> DSLDEQRSRYAQIKQAWDNRQMDVVEQMMPGLKDYPLYPYLEYRQITDDLMNQPAVTVTNFVRANPTLPPARTLQSRFVNELARREDWRGLLAFSPEKPGTT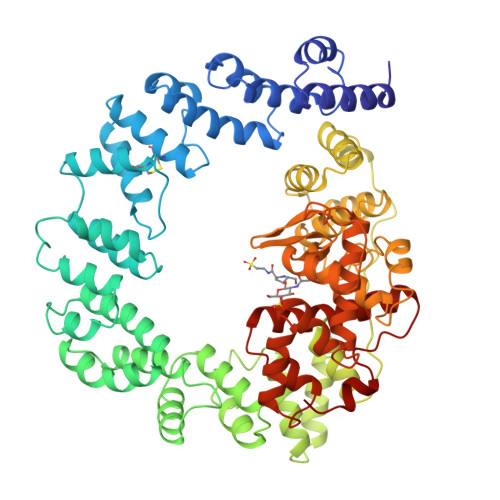EAQCNYYYAKWNTGQSEEAWQGAKELWLTGKSQPNACDKLFSVWRASGKQDPLAYLERIRLAMKAGNTGLVTVLAGQMPADYQTIASAIISLANNPNTVLTFARTTGATDFTRQMAAVAFASVARQDAENARLMIPSLAQAQQLNEDQIQELRDIVAWRLMGNDVTDEQAKWRDDAIMRSQSTSLIERRVRMALGTGDRRGLNTWLARLPMEAKEKDEWRYWQADLLLERGREAEAKEILHQLMQQRGFYPMVAAQRIGEEYELKIDKAPQNVDSALTQGPEMARVRELMYWNLDNTARSEWANLVKSKSKTEQAQLARYAFNNQWWDLSVQATIAGKLWDHLEERFPLAYNDLFKRYTSGKEIPQSYAMAIARQESAWNPKVKSPVGASGLMQIMPGTATHTVKMFSIPGYSSPGQLLDPETNINIGTSYLQYVYQQFGNNRIFSSAAYNAGLGRVRTWLGNSAGRIDAVAFVESIPFSETRGYVKNVLAYDAYYRYFMGDKPTLMSATEWGRRY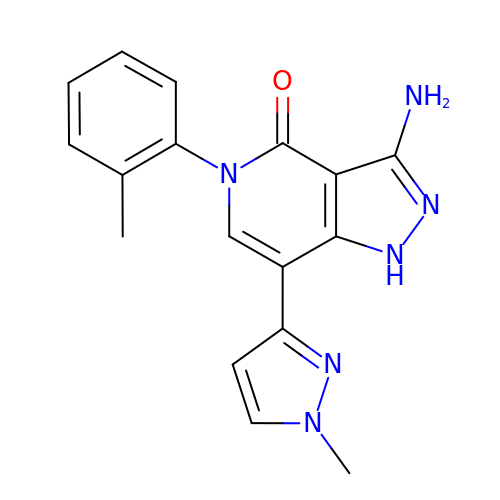3-azanyl-5-(2-methylphenyl)-7-(1-methylpyrazol-3-yl)-1~{H}-pyrazolo[4,3-c]pyridin-4-one | C17 H16 N6 O | VVMMTCDXQMWVBF-UHFFFAOYSA-N>[4x]MIKKNKADFTSNGSNNKAISTVEPHYEDTAPAEKVIKSLTSISPPGVEPMMPGSDKTPKNRNEKLTQLDKFRFAPQGESLRTNQGVKISDNQNSLKSGARGSTLLEDFILREKITHFDHERIPERVVHARGTGAHGYFQVYESLASYTTAEFLQDPSVKTPVFVRFSTVQGSRGSADTVRDIRGWATKFYTKEGTFDLVGNNTPVFFIQDAIKFPDFVHAVKPEPHNEIPQGQSA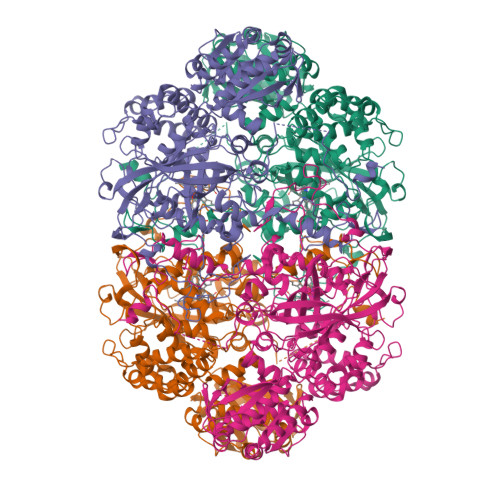HDTFWDYISLQPETLHNVMWVMSDRGIPRSYRMMEGFGIHTYKMINAEGQCHFIRFHWKPVYGVSSLIWDEAQLLTGCDPDFHRRELWESIEAGDYPEYELGLQIIPEEDEHKFDFDILDPTKLIPESLVPVHLVGKMVLNRNPDNYFSETEQVAFCPGNIVPGIDFSDDPLLQGRLFSYIDTQISRLGGVNFHEIPINKPICPFHNHQRDGMHRMSISGTANYEPNSINNNWPREAPPTEGGFTTYPQPVNGYKSRKRSSTFIDFYSQPRLFWLSQTKVEQNHIVGGFSFELGKVVRPWIRERVVNQLTYIDHQLAQSVADNLGIKLSQEQLKHPLPGPINGLSKDRSLSMYDGHHQILKSRQVAILAADGVCGDAIDNIMKTLKKYGVHGKIFAPHVGRITSLQGNEIEVNGTIEGNPSVMVDAVIIPDGEDSIDSLMKNGNAKHYVIQAFKHLKAIGLQGKAFKLYDALPLPKPDEGIVVGDKAADLAEAFCNVMRGHRIWSRESVAQEIAG> VRPWSEFRLTPAEAAAAAALAARCAQRYDETDGPEFLLDAPVIAHELPRRLRTFMARARLDAWPHALVVRGNPVDDAALGSTPVHWRTARTPGSRPLSFLLMLYAGLLGDVFGWATQQDGRVVTDVLPIKGGEHTLVSSSSRQELGWHTEDAFSPYRADYVGLLSLRNPDGVATTLAGVPLDDLDERTLDVLFQERFLIRPDDSHLQVNNSTAQQGRVEFEGIAQAADRPEPVAILTGHRAAPHLRVDGDFSAPAEGDEEAAAALGTLRKLIDASLYELVLDQGDVAFIDNRRAV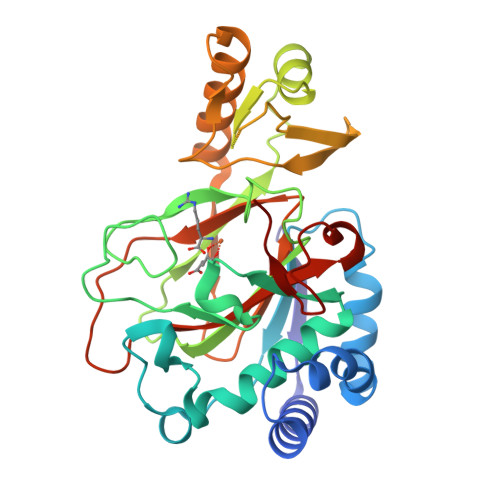HGRRAFQPRYDGRDRWLKRINITRDLHRSRKAWAGDSRVLGQR>[4x]GAMASGKVVKFSYMWTINNFSFCREEMGEVIKSSTFSSGAND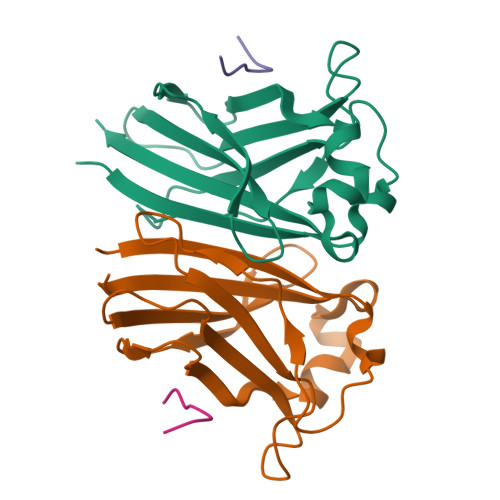KLKWCLRVNPKGLDEESKDYLSLYLLLVSCPKSEVRAKFKFSILNAKGEETKAMESQRAYRFVQGKDWGFKKFIRRNFLLDEANGLLPDDKLTLFCEVSVVQD;>KADTTTPTT[4x]>[2x]ENLYFQGAMELIEQHQIFGGSQQVWAHHAQTLQCEMKFAVYLPNNPENRPLGVIYWLSGLTCTEQNFITKSGFQRYAAEHQVIVVAPDTSPRGEQVPNDDAYDLGQSAGFYLNATEQPWAANYQMYDYILNELPRLIEKHFPTNGKRSIMGHSMGGHGALVLALRNQERYQSVSAF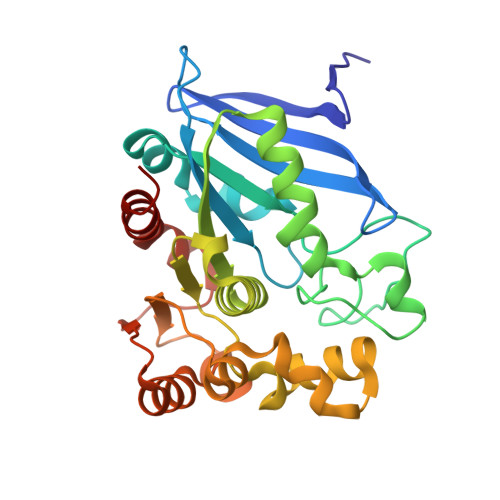SPILSPSLVPWGEKAFTAYLGKDREKWQQYDANSLIQQGYKVQGMRIDQGLEDEFLPTQLRTEDFIETCRAANQPVDVRFHKGYDHSYYFIASFIGEHIAYHAAFLK>[2x]ATDDVSKAYSSPTFDAEALLGTVISAEDPDRVLIEPWATGVDGVILDVGSGTGRWTGHLASLGHQIEGLEPATRLVELARQTHPS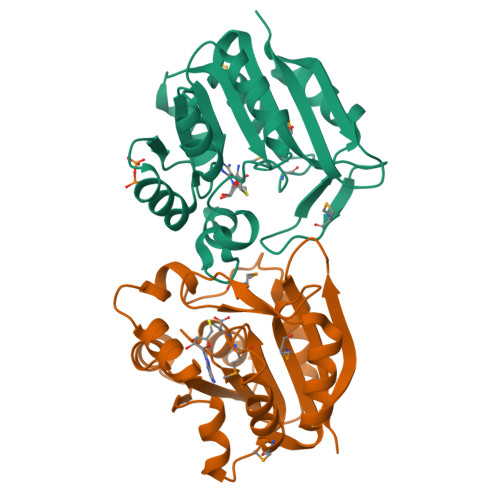VTFHHGTITDLSDSPKRWAGLLAWYSLIHMGPGELPDALVALRMAVEDGGGLLMSFFSGPSLEPMYHPVATAYRWPLPELAQALETAGFQVTSSHWDPRFPHAYLTAEASLEHHHHHH>[2x]SSPLPLVVNTWPFKNATEAAWRALASGGSALDAVESGCAMCEREQCDGSVGFGGSPDELGETTLDAMIMDGTTMDVGAVGDLRRIKNAIGVARKVLEHTTHTLLVGESATTFAQSMGFINEDLSTSASQALHSDWLARNCQPNYWRNVIPDPSKYCGPYKPP;>TIGMVVIHKTGHIAAGTSTNGIKFK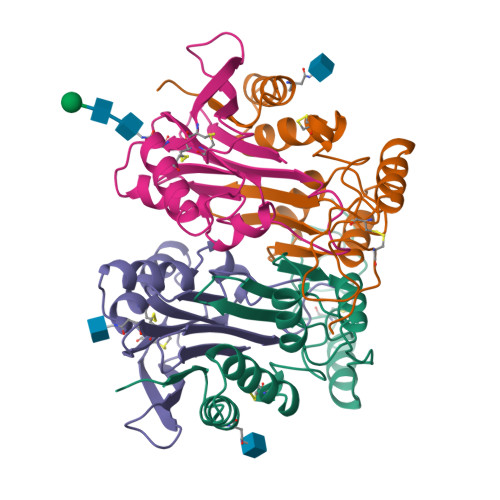IHGRVGDSPIPGAGAYADDTAGAAAATGNGDILMRFLPSYQAVEYMRRGEDPTIACQKVISRIQKHFPEFFGAVICANVTGSYGAACNKLSTFTQFSFMVYNSEKNQPTEEKVDCI[2x]> VKVDLESKRYGEKLKEVFLMLDNNVVECIKEITESSRNGKLVFFVGAGVSTLSDYPQWWRLVDKYHEELYGSPKKGNYSSDEYLRIPQIFYNVKGEMAFDGILKDFFQVDKPTNPIHDKILAMNPAHVITTNYDNLIDTACWKRGKYFSVISAEEDVANATSSRYLLKVAGDFRKGFKGENVVLKEDDYLNYDQNYPLISNLMKTIIATHTIVFIGYGLGDYNINMLLNWVRKLQKDSFHKPFFIRTDPSPIENETLIYYENK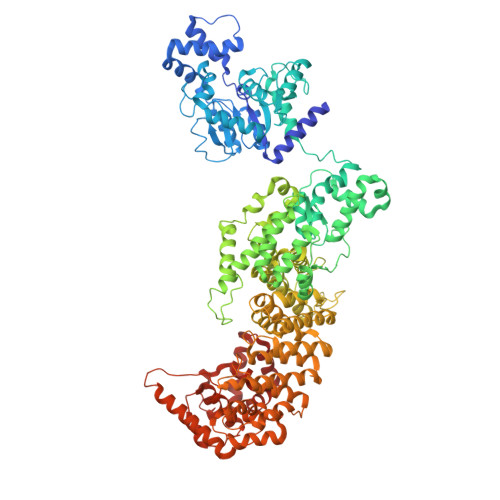GLRIIDAASLIDSNEYDYLERYSAVMDLLIESQENKFITKDDEVIDYIYGKISPLFALQYIRKIDLKHVFEYDYHFEVNGTVVRHKNKGFGYMERFFELKESCDERSKLSKKQYERFNALFNFFEKNGVICMAKDAGTLNTSIEINSLAYHGKYDVMKKFIEEQSVSIEDDYKKAFFLACLGRWEESYDLYSNIILNSIDESNGCVYYLSQINRYRIYQSITQAVTQFNGLGLLTFGRHYKPFTDEFLARIEREMTNFNIDDLFNGMPFEFQKKYKILEFLSDNQFLYDDTVKLFELTNKVRSEMSEGSYSFGMSSDIVVLLRLYDNLRFLYENCLWSVSFHEFHQYIRNSMSLLIEKAEYERTRDIDELGFSFFGKKSGFFMEYYDFVNISRHFKIDDIKNLERSCSIDKIRFGEQEKIEEYLVGIAEEITKQFSANGMNVVFYTQFISEAKAALYFAKYVKLSEEGLGKIVKALLFYFPERDLDIGKRYVWLERLTKCNELPKSIISIIDDFLVLQAEKHIDQNYSEVSSNGLYSRDYGALIKHFEKNFISKRLSEITLCLTQDKQKQIDFLFKLLPLLSTNAKSHLLSFKSVENINDLMNGIRIGLIDEFTPEHEELIIEYLETRKVNYIVEKEKGIQTFSSNDYMSTFGIWYFLEEINNSKMEEFIGMDDQYDFFVDPENFDYKKFIPSWLKNYNDKLLGKIAGNKHMKHHVIEVLKERVKNSNDKRYLEILMNYFI> MGESQTLDKVYQMKSKPRGYCLIINNHNFAKAREKVPKLHSIRDRNGTHLDAGALTTTFE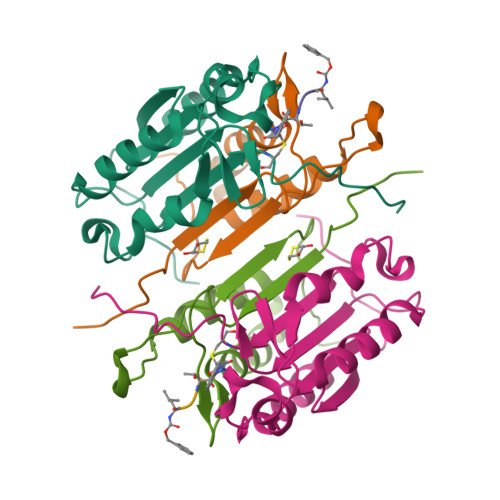ELHFEIKPHDDCTVEQIYEILKIYQLMDHSNMDCFICCILSHGDKGIIYGTDGQEAPIYELTSQFTGLKCPSLAGKPKVFFIQACQGDNYQKGIPVETD;> MAEEQPYLEMDLSSPQTRYIPDEADFLLGMATVNNCVSYRNPAEGTWYIQSLCQSLRERCPRGDDILTILTEVNYEVSNKDDKKNMGKQMPQPTFTLRKKLVFPSD> GSVGPKTGEENQVLVPNLNPTPENLEVVGDGFKITSSINLVGEEEADENAVNALREFLTANNIEINSENDPNSTTLIIGEVDDDIPELDEALNGTTAENLKEEGYALVSNDGKIAIEGKDGDGTFYGVQTFKQLVKESNIPEVNITDYPTVSARGIVEGFYGTPWTHQDRLDQIKFYGENKLNTYIYAPKDDPYHREKWREPYPESEMQRMQELINASAENKVDFVFGISPGIDIRFDGDAGEEDFNHLITKAESLYDMGVRSFAIYWDNIQDKSAAKHAQVLNRFNEEFVKAKGDVKPLITVPTEYDTGAMVSNGQPRAYTRIFAETVDPSIEVMWTGPGVVTNEIPLSDAQLISGIYDRNMAVWWNYPVTDYFKGKLALGPMHGLDKGLNQYVDFFTVNPMEHAELSKISIHTAADYSWNMDNYDYDKAWNRAIDMLYGDLAEDMKVFANHSTRMDNKTWAKSGREDAPELRAKMDELWNKLSSKEDASALIEELYGEFARMEEACNNLKANLPEVALEECSRQLDELITLAQGDKASLDMIVAQLNEDTEAYESAKEIAQN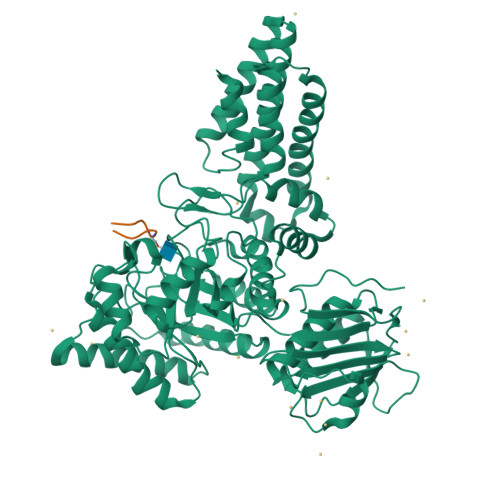KLNTALSSFAVISEKVAQSFIQEALS;> QLWVDSTPPPG>[2x]LRLPRETDE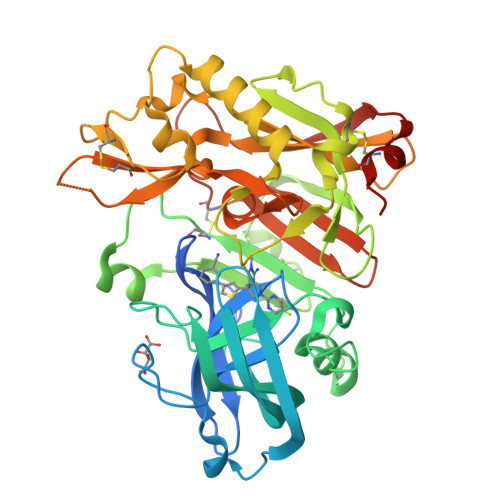EPEEPGRRGSFVEMVDNLRGKSGQGYYVEMTVGSPPQTLNILVDTGSSNFAVGAAPHPFLHRYYQRQLSSTYRDLRKGVYVPYTQGKWEGELGTDLVSIPHGPNVTVRANIAAITESDKFFINGSNWEGILGLAYAEIARPDDSLEPFFDSLVKQTHVPNLFSLQLCGAGFPLNQSEVLASVGGSMIIGGIDHSLYTGSLWYTPIRREWYYEVIIVRVEINGQDLKMDCKEYNYDKSIVDSGTTNLRLPKKVFEAAVKSIKAASSTEKFPDGFWLGEQLVCWQAGTTPWNIFPVISLYLMGEVTNQSFRITILPQQYLRPVEDVATSQDDCYKFAISQSSTGTVMGAVIMEGFYVVFDRARKRIGFAVSACHVHDEFRTAAVEGPFVTLDMEDCGYNIPQTDEST>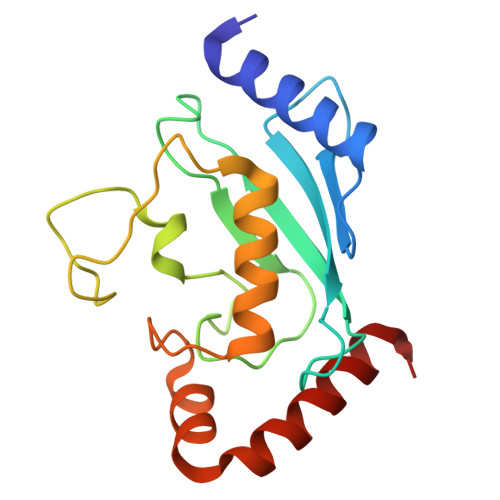 AGTALKRLMAEYKQLTLNPPEGIVAGPMNEENFFEWEALIMGPEDTCFEFGVFPAILSFPLDYPLSPPKMRFTCEMFHPNIYPDGRVCISILHAPGDDPMGYESSAERWSPVQSVEKILLSVVSMLAEPNDESGANVDASKMWRDDREQFYKIAKQIVQKSLGL L‐Asparaginases (ASNases) catalyze the hydrolysis of L‐Asn to L‐Asp and ammonia. In contrast, the chain of ASNase from Rhodospirillum rubrum, reported here and referred to as RrA, consists of only 172 amino acid residues. RrA is homologous to the N‐terminal domain of typical bacterial class 1 ASNases and exhibits millimolar affinity for L‐Asn. Crystal structures of the wild‐type RrA, both with and without bound L‐Asp, as well as structures of several RrA mutants, reveal topologically unique tetramers.

A distinctive feature of RrA is the presence of Lys19 within the lining of the substrate‐binding site. We probed the importance of this residue by mutating it to L‐Ala, L‐Glu, and L‐Gln. Crystals of RrA(K19A) obtained in the absence of L‐Asp were also isomorphous with those of RrA(K19Q). The region 58–62 of the main chain of protomer A of RrA(K19A) is disordered. However, the main chain adjacent to the mutation site is well ordered in both protomers, and the area occupied by the side chain of Lys19 in the native protein appears occupied only by water molecules. The kinetic data, even when reduced to approximate turnover numbers, demonstrate that Lys19 plays an important role during catalysis and its mutation reduces the rate of catalysis by two or more orders of magnitude.

>[2x]HHHHHHENLYFQSMAVSPSPLRIFTAGGTIDADYRLEENGLVVGDPFVAEVLKTARLAGAVSIVALSRKDSLDFTEADREAIGRAVGQAVEDHILLTHGTDTMVETARYLGGLPELAGKTVVLSGAMVPGRVGGSDAAFNIGFACAAALMLAPGVYIAMHGKVFDPAKTRKNRGLGRFEPIDDQE>[3x]GPTNFEKEYDLEKLVNNSLDLLSIQRLDGTVLQVNPAFERLLGWREEELIG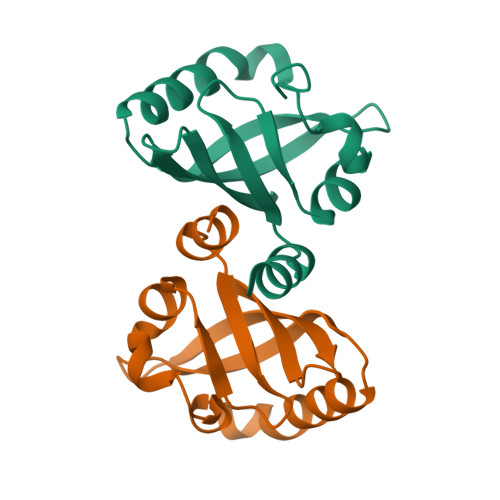RNPFHLLHPEDRESTFQEFKKLNQGLPVFAFQNRFLCSDGTYKYFSWTASPDLSAGLIYVTGRDI> GSPESFPDAHMRMILRKPPGQRTVDDLEIIYDELLHIKALSHLSTTVKRELAGVLIFESHAKGGTVLFNQGEEGTSWYIILKGSVNVVIYGKGVVCTLHEGDDFGKLALVNDAPRAASIVLREDNCHFLRVDKEDFNRILRDVEANTVRLKEHDQDVLVLEKVPAGNRAANQGNSQPQQKYTVMSGTPEKILEHFLETIRLEPSLNEATDSVLNDFVMMHCVFMPNTQLCPALVAHYHAQPSQGTEQERMDYALNNKRRVIRLVLQWAAMYGDLLQEDDVAMAFLEEFYVSVSDDARMMAAFKEQLPELEKIVKQISEDAKAPQKKHKVLLQQFNTGDERAQKRQPIRGSDEVLFKVYCIDHTYTTIRVPVAASVKEVISAVADKLGSGEGLIIVKMNSGGEKVVLKSNDVSVFTTLTINGRLFACPREQFDSLTPLPEQEGPTTGTVGTFELMSSKDLAYQMTTYDWELFNCVHELELIYHTFGRHNFKKTTANLDLFLRRFNEIQFWVVTEVCLCSQLSKRVQLLKKFIKIAAHCKEYKNLNSFFAIVMGLSNVAVSRLALTWEKLPSKFKKFYAEFESLMDPSRNHRAYRLTAAKLEPPLIPFMPLLIKDMTFTHEGNKTFIDNLVNFEKMRMIANTARTVRYYRSQPFNPDAAQANKNHQDVRSYVRQLNVIDNQRTLSQMSHRLEPRRP;> MREYKLVVLGSGGVGKSALTVQFVQGIFVEKYDPTIEDSYRKQVEVDAQQCMLEILDTAGTEQFTAMRDLYMKNGQGFALVYSITAQSTFNDLQDLREQILRVKDTDDVPMILVGNKCDLEDERVVGKEQG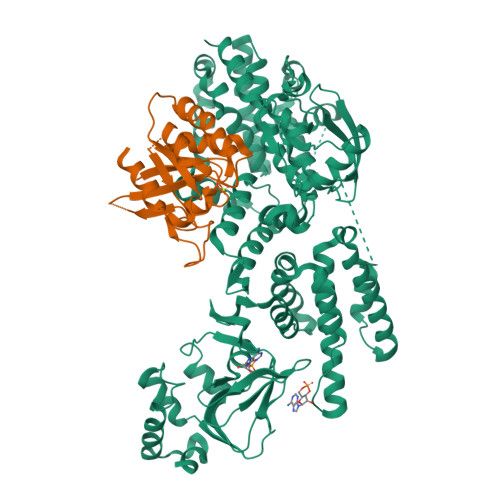QNLARQWNNCAFLESSAKSKINVNEIFYDLVRQINR> MGSVTPIPLPKIDEPEEYNTNYILFWNHVGLELNRVTHTVGGPLTGPPLSARALGMLHLAIHDAYFSICPPTDFTTFLSPDTENAAYRLPSPNGANDARQAVAGAALKMLSSLYMKPVEQPNPNPGANISDNAYAQLGLVLDRSVLEAPGGVDRESASFMFGEDVADVFFALLNDPRGASQEGYHPTPGRYKFDDEPTHPVVLIPVDPNNPNGPKMPFRQYHAPFYGKTTKRFATQSEHFLADPPGLRSNADETAEYDDAVRVAIAMGGAQALNSTKRSPWQTAQGLYWAYAGSNLIGTPPRFYNQIVRRIAVTYKKEEDLANSEVNNADFARLFALVDVACTDAGIFSWKEKWEFEFWRPLSGVRDDGR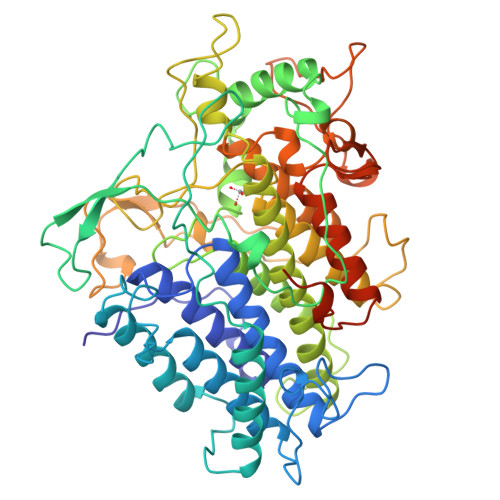PDHGDPFWLTLGAPATNTNDIPFKPPFPAYPSGHATFGGAVFQMVRRYYNGRVGTWKDDEPDNIAIDMMISEELNGVNRDLRQPYDPTAPIEDQPGIVRTRIVRHFDSAWELMFENAISRIFLGVHWRFDAAAARDILIPTTTKDVYAVDNNGATVFQNVEDIRYTTRGTREDEEGLFPIGGVPLGIEIADEIFNNGLKPTPPEIQPMPQETPVQKPVGQQPVKGMWEEEQAPVVKEAP> GPPYCVFPGRRTSSTSFTTSFST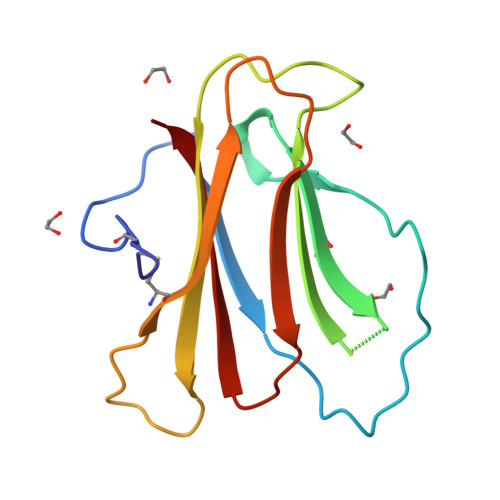EPLGYARMLHRDPPYERAGNSGLNHRIYERSRVGGLRTVIDVAPPDGHQAIANYEIEVRRIPVATPNAAGDCFHTARLSTGSRGPATISWDADASYTYYLTISED>[4x]MDYKDDDDKMAGKR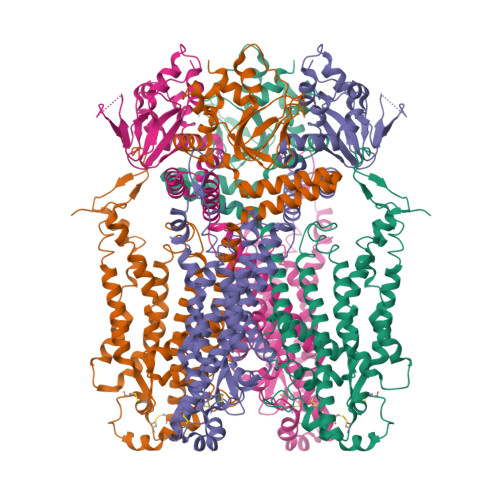ENFVRVDDLDSRLPSSSVAFQQNYASNFSGQLHPIHASNETSRSFKKGIQKGSKGLKSIGRSLGFGVYRAVFPEDLKVSEKKIFDPQDKFLLYCNKLFVASCILSVFVDPFFFYLPVINAESKCLGIDRKLAITASTLRTFIDVFYLAHMALQLRTAYIAPSSRVFGRGELVIDPAQIAKRYLQRWFIIDFLSVLPLPQIVVWRFLQSSNGSDVLATKQALLFIVLVQYIPRFLRVLPLTSELKRTAGVFAETAWAGAAYYLLLYMLASHIVGAFWYLLALERNDACWQEACIDAGNCSTDFLYCGNQNMDGYAVWNRAKESVLKSKCRADLDDNNPPFDFGIYTQALSSGIVSSQNFIVKYCYCLWWGLQNLSTLGQGLETSTYPMEIIFSISLAISGLILFALLIGNMQTYLQSLTIRLEEMRVKRRDSEQWMHHRMLPQDLRERVRRYDQYKWLETRGVDEEYLVQNLPKDLRRDIKRHLCLALVRRVPLFKSMDDKLLDAICMRLKPCLFTESTYLVREGDPVDEMLFIIRGRLESVTTDGGRSGFFNRSLLKEGEFCGEELLTWALDPKSGVNLPSSTRTVKALTEVEAFALTSEELKFVASQFRRLHSRQVQHTFRFYSHQWRTWAACFIQAAWRRYCKRKKMEEAEAEAAAVSSSTAGPSYSIGAAFLATKFAANALRTIHRNRNTKIRDLVKLQKPPEPDFTAD N-(4-{4-[1-(cyclopropylsulfonyl)cyclopropyl]-6-[(3S)-3-methylmorpholin-4-yl]pyrimidin-2-yl}phenyl)-N'-(2-hydroxyethyl)thiourea | C24 H31 N5 O4 S2 | 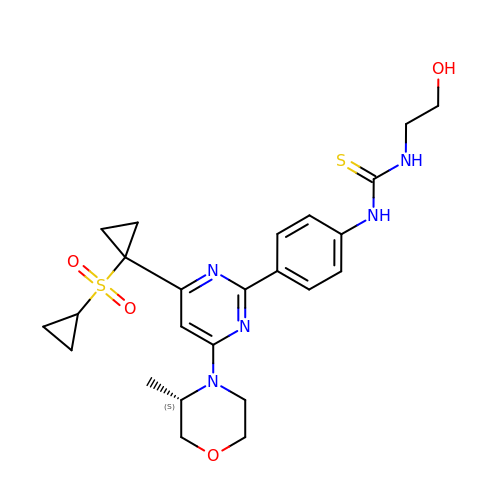JWGVUDPAMQEIJU-INIZCTEOSA-N>[4x]SEGSDAPNFVLEDTNGKRIELSDLKGKGVFLNFWG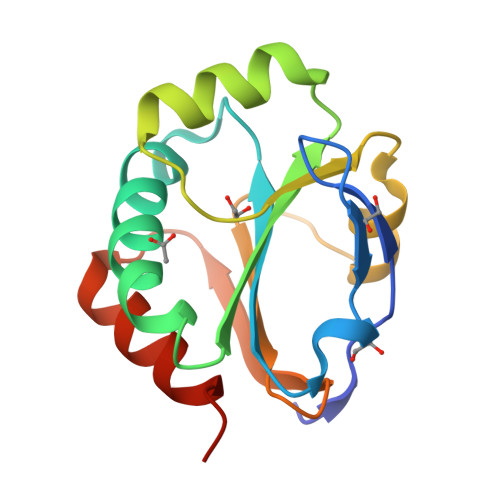TWCEPCKKQFPYMANQYKHFKSQGVEIVAVNVGESKIAVHNFMKSYGVNFPVVLDTDRQVLDAYDVSPLPTTFLINPEGKVVKVVTGTMTESMIHDYMNLIKPGETSG Peptides destined for display are first delivered into the endoplasmic reticulum (ER) by the transporter associated with antigen processing (TAP). TAP is a heteromeric ATP-binding cassette (ABC) transporter comprising two subunits, TAP1 and TAP2. Each subunit has an N-terminal transmembrane domain (TMD0) that interacts with other components of the larger peptide-loading complex, a six-transmembrane helical domain (TMD) that forms the translocation pathway, and a nucleotide-binding domain (NBD) that hydrolyzes ATP. In this study, we analyzed the structure of TAP in the presence and absence of peptides. These structures show that TAP suspends peptides across its transmembrane cavity, anchoring their termini in two distal binding pockets primarily through their backbone atoms.

To understand how TAP recognizes peptide antigens, we analyzed the structures of TAP in complex with b27 and two other 9-mer peptides, all of which have optimal lengths for binding. These three peptides, b27, ILKEPVHGV (a2), and QYDDAVYKL (c4), are natural products of the antigen processing pathway and are presented by HLA-B27, HLA-A2, and HLA-C4, respectively. The structures of a2- and c4-bound TAP are essentially identical, having an overall rmsd of 0.8 Å. Nevertheless, the peptides are suspended in a central cavity surrounded by TMs 2-6 from both TAP1 and TAP2 in all three structures. When viewed from a perspective perpendicular to the membrane plane, each peptide stretches roughly 27 Å across the TM cavity. Despite their sequence diversity, the three 9-mer peptides are stabilized in the peptide-binding pocket by a common set of interactions involving backbone atoms on each end of the peptide. These interactions, including eight hydrogen bonds, a cation-π, and two van der Waals interactions, enable sequence-independent binding to TAP. At the N-terminal region, the free amino group of each peptide forms a cation-π interaction with TAP1 W308 and two hydrogen bonds with TAP1 E242 and D246. The terminal carboxyl group of all three peptides forms hydrogen bonds with TAP2 N269 and R273, as well as longer-range electrostatic interactions with TAP2 R210. Furthermore, TAP2 L377 forms van der Waals interactions with the N terminus of all three peptides, and R373 interacts with the main chain atoms of a2 and c4 but not b27.

> MASSRCPAPRGCRCLPGASLAWLGTVLLLLADWVLLRTALPRIFSLLVPTALPLLRVWAVGLSRWAVLWLGACGVLRATVGSKSENAGAQGWLAALKPLAAALGLALPGLALFRELISWGAPGSADSTRLLHWGSHPTAFVVSYAAALPAAALWHKLGSLWVPGGQGGSGNPVRRLLGCLGSETRRLSLFLVLVVLSSLGEMAIPFFTGRLTDWILQDGSADTFTRNLTLMSILTIASAVLEFVGDGIYNNTMGHVHSHLQGEVFGAVLRQETEFFQQNQTGNIMSRVTEDTSTLSDSLSENLSLFLWYLVRGLCLLGIMLWGSVSLTMVTLITLPLLFLLPKKVGKWYQLLEVQVRESLAKSSQVAIEALSAMPTVRSFANEEGEAQKFREKLQEIKTLNQKEAVAYAVNSWTTSISGMLLKVGILYIGGQLVTSGAVSSGNLVTFVLYQMQFTQAVEVLLSIYPRVQKAVGSSEKIFEYLDRTPRCPPSGLLTPLHLEGLVQFQDVSFAYPNRPDVLVLQGLTFTLRPGEVTALVGPNGSGKSTVAALLQNLYQPTGGQLLLDGKPLPQYEHRYLHRQVAAVGQEPQVFGRSLQENIAYGLTQKPTMEEITAAAVKSGAHSFISGLPQGYDTEVDEAGSQLSGGQRQAVALARALIRKPCVLILDDATSALDANSQLQVEQLLYESPERYSRSVLLITQHLSLVEQADHILFLEGGAIREGGTHQQLMEKKGCYWAMVQAPADAPE;> MRLPDLRPWTSLLLVDAALLWLLQGPLGTLLPQGLPGLWLEGTLRLGGLWGLLKLRGLLGFVGTLLLPLCLATPLTVSLRALVAGASRAPPARVASAPWSWLLVGYGAAGLSWSLWAVLSPPGAQEKEQDQVNNKVLMWRLLKLSRPDLPLLVAAFFFLVLAVLGETLIPHYSGRVIDILGGDFDPHAFASAIFFMCLFSFGSSLSAGCRGGCFTYTMSRINLRIREQLFSSLLRQDLGFFQETKTGELNSRLSSDTTLMSNWLPLNANVLLRSLVKVVGLYGFMLSISPRLTLLSLLHMPFTIAAEKVYNTRHQEVLREIQDAVARAGQVVREAVGGLQTVRSFGAEEHEVCRYKEALEQCRQLYWRRDLERALYLLVRRVLHLGVQMLMLSCGLQQMQDGELTQGSLLSFMIYQESVGSYVQTLVYIYGDMLSNVGAAEKVFSYMDRQPNLPSPGTLAPTTLQGVVKFQDVSFAYPNRPDRPVLKGLTFTLRPGEVTALVGPNGSGKSTVAALLQNLYQPTGGQVLLDEKPISQYEHCYLHSQVVSVGQEPVLFSGSVRNNIAYGLQSCEDDKVMAAAQAAHADDFIQEMEHGIYTDVGEKGSQLAAGQKQRLAIARALVRDPRVLILDEATSALDVQCEQALQDWNSRGDRTVLVIAHRLQTVQRAHQILVLQEGKLQKLAQL;> ILKEPVHGV> GGGSGAAAPRRCLLSHYRSLEPRTLAAAKALRDRYEEEALSWGQRNCSFRPRRDPPRPSSCARLRHVARGIADAQAVLSGLHRSELLPGAGPILELLAAAGRDVAACLELARPGSSRKVPGAQKRRHKPRRADSPRCRKASVVFN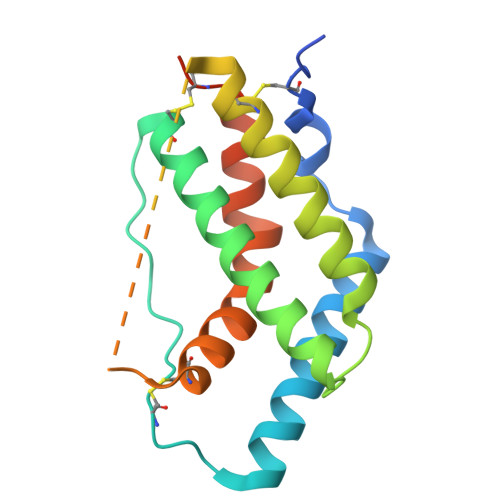LLRLLTWELRLAAHSGPCLAAAHHHHHHHH> ATGGYVQQATGQASFTMYSGCGSPACGKAASGFTAAINQLAFGSAPGLGAGDACGRCFALTGNHDPYSPNYTGPFGQTIVVKVTDLCPVQGNQEFCGQTTSNPTNQHGMPFHFDICEDTGGSAKFFPSGHGALT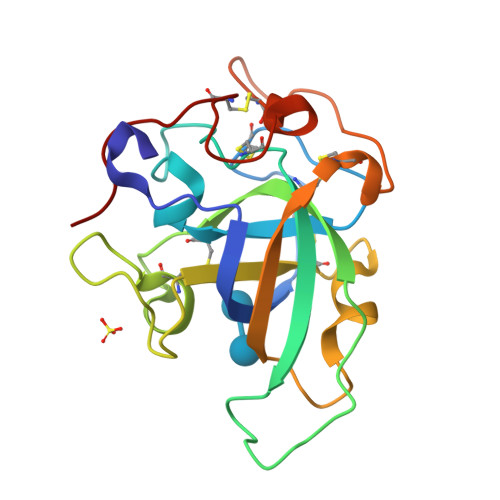GTFTEVSCSQWSGSDGGQLWNGACLSGETAPNWPSTACGNKGTAPS>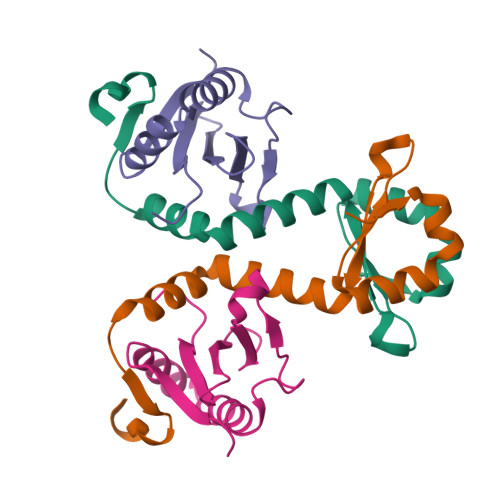[2x]MIITSPTEARKDFYQLLKNVNNNHEPIYISGNNAENNAVIIGLEDWKSIQETIYLESTGTMDKVREREKDNSGTTNIDDIDWDNL;>MSNYTVKIKNSAKSDLKKIKHSYLKKSFLEIVETLKNDPYKITQSFEKLEPKYLERYSRRINHQHRVVYTVDDRNKEVLILSAWSHYD[2x]> GMNDRKILVAYFSCSGVTKAVAEKLAAITGADLYEIKPEVPYTEADLDWNDKKSRSSVEMRDALSRPAISGTLFHPEKYEVLFVGFPVWWYIAPTIINTFLESYDFAGKIVVPFATSGGSG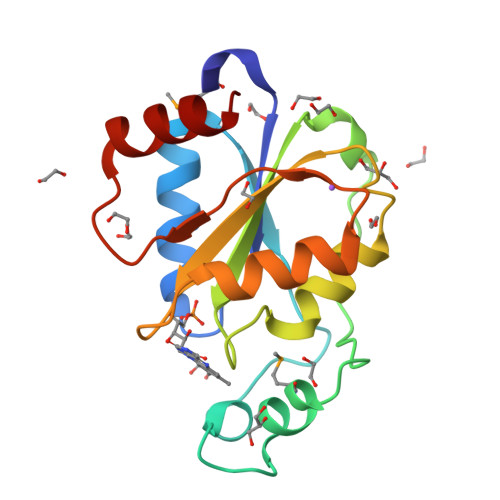IGNCEKNLHKAYPDIVWKDGKLLNGQITRDLVTEWFEKIRL>[2x]MAEPWGNELASAAARGDLEQLTSLLQNNVNVNAQNGFGRTALQVMKLGNPEIARRLLLRGA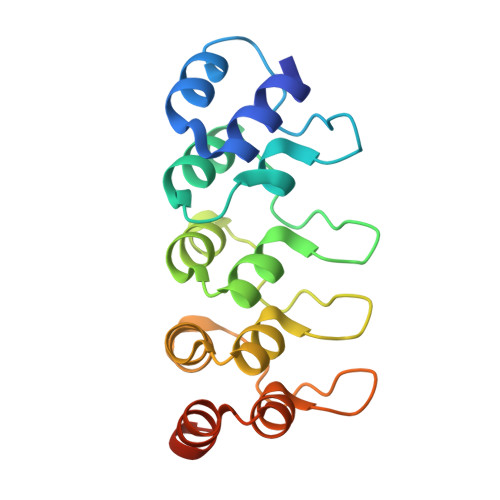NPDLKDRTGNAVIHDAARAGFLDTLQTLLEFQADVNIEDNEGNLPLHLAAKEGHLRVVEFLVKHTASNVGHRNHKGDTACDLARLYGRNEVVSLMQANGAGGATNLQ> MGSSHHHHHHGSGVKTENNDHINLKVAGQDGSVVQFKIKRHTPLSKLMKAYCERQGLSMRQIRFRFDGQPINETDTPAQLEMEDEDTIDVFQQQTGGSKFSNITIKNFRNFEKVNINLDNKNVIFGMNDIGKTNFLYALRFLLDKEIRKFGFNKSDYHKHDTSKKIEIILTLDLSNYEKDEDTKKLISVVKGARTSANADVFYIALESKYDDKELYGNIILKWGS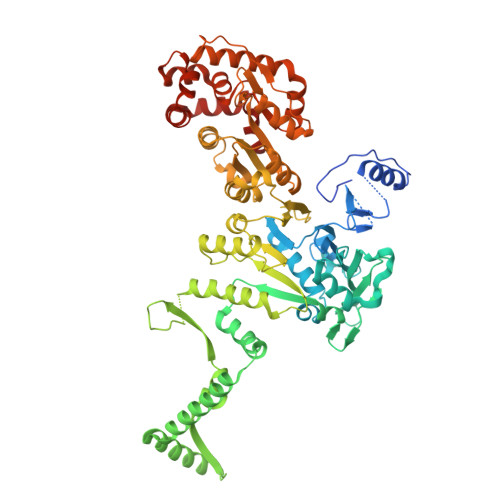ELDNLIDIPGRGNINALDNVFKVIYINPLVDLDKLFAQNKKYIFEESQGNESDEGILNNIKSLTDQVNQQIGEMTIIKGFQQEITSEYRSLKKEEVSIELKSEMAIKGFFSDIIPYIKKDGDSNYYPTSGDGRRKMLSYSIYNYLAKKKYEDKIVIYLIEEPEISLHRSMQIALSKQLFEQSTYKYFFLSTHSPELLYEMDNTRLIRVHSTEKVVCSSHMYNVEEAYGSVKKKLNKALSSALFAERVLLIEGPSEKILFEKVLDEVEPEYELNGGFLLEVGGTYFNHYVCTLNDLGITHIIKTDNDLKSKKGKKGVYELLGLNRCLNLLGRENLDEITIDIPEDIKGKKKKERLNERKKEIFKQYKNEVGEFLGERIYLSEIDLENDLYSAIGESMKRIFENEDPVHYLQKSKLFNMVELVNNLSTKDCFDVFEHEKFACLKELVGSDRG>[2x]MNTKYNKEFLLYLAGFVDGDGSIIAQIKPNQSYKFKHQLSLTFQVTEKTQRRWFLDKLVDEIGVGYVRDRGSVSDYILSEIKPLHNFLTQLQPFLKL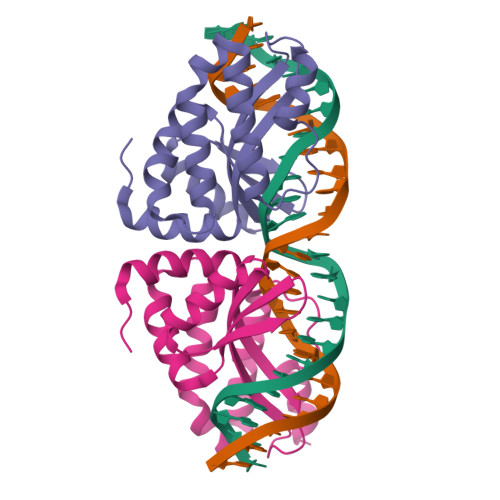KQKQANLVLKIIEQLPSAKESPDKFLEVCTWVDQIAALNDSKTRKTTSETVRAVLDSLSEKKKSSP>DGAEREAALERPRRTKRERDQLYYECYSDVSVHEEMIADRVRTDAYRLGILRNWAALRGKTVLDVGAGTGILSIFCAQAGARRVYAVEASAIWQQAREVVRFNGLEDRVHVLPGPVETVELPEQVDAIVSEWMGYGLLHESMLSSVLHARTKWLKEGGLLLPASAELFIAPISDQMLEWRLGFWSQVKQHYGVDMSCLEGFATRCLMGHSEIVVQGLSGEDVLAR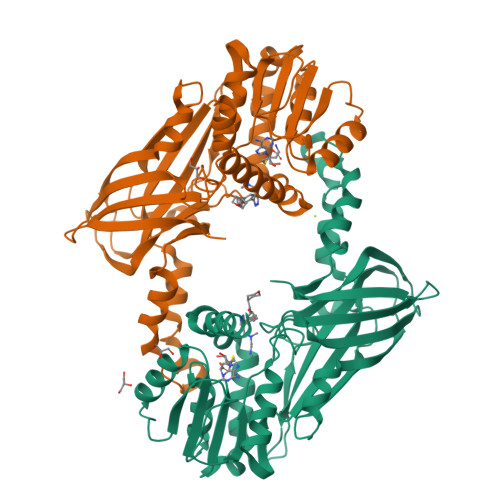PQRFAQLELSRAGLEQELQAGVGGRFRCSCYGSAPMHGFAIWFQVTFPGGESEKPLVLSTSPFHPATHWKQALLYLNEPVQVEQDTDVSGEITLLPSRDNPRRLRVLLRYKVGDQEEKTKDFAMED[2x]>LDRADILYNIRQTSRPDVIPTQRDRPVAVSVSLKFINILEVNEITNEVDVVFWQQTTWSDRTLAWNSSHSPDQVSVPISSLWVPDLAAYNAISKPEVLTPQLARVVSDGEVLYMPSIRQRFSCDVSGVDTESGATCRIKIGSWTHHSREISVDPTTENSDDSEYFSQYSRFEILDVTQKK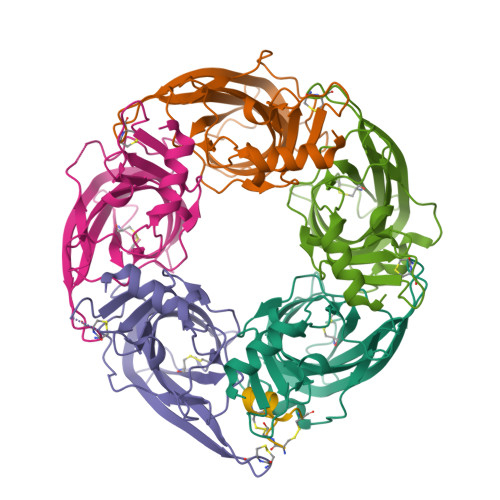NSVTYSCCPEAYEDVEVSLNFRKKG[5x];> SCCARNPACRHNHPCV> MAPTPKYTFTERAAAGNLSDAEILNSNN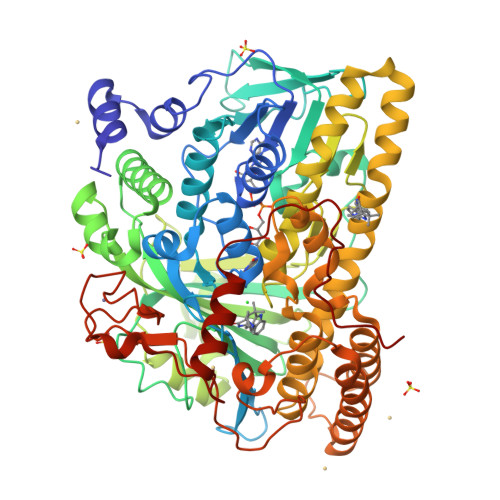PTGSELPDESDVVVGGAGIHGLIYALHASKYKPNNLKISVIEKNTRPGYKIGESTLPIFYTWCKLHGISAAYLLRLFGLKDGLCFYFLDRENQGQYTDFCSVGAPGLVLASLQIERPMSELLFTILAQRNGVNVYHGREVDFKSTVVQGGGQGNKIAVSRGKYDSTPKTIDSALFVDATGRFRQFCSKKAPRHRFDGWNCNAFWGYFTAPKDESKIPFDLYEGDATNHLCFPEGWVWVIRLPSWEGSPIANLMDMVTYILECADAGVPGDELPSSEELARMFGLKFQWVTSIGFAVRNDVKYPEDLSAYGTREAEQKFNYFVQKYELLQQFMSNFELIENLYGPGTTWFIRKTLAYQSPVVSGPGWLAIGDACGFTNPLYSPGINVGMSTSTWAAQLSHPIVEIGKSAPADAAESSIRKLLVPYDDYCKSLVPALEQMNRFNYVCYRDTRLGPQVACLWQFFAGIERYLSDVNIETFAHYAIKWVWGAMVPEYQQVAQKCIEHIETVPLDERLPDAMVDELLAFSNRIKSAAVAADDFSLRWDAILRSFDRSLNFVEGKTSRDIYTRQCSGCGAWLQLRPDWKKCHSCGLLGTEPQTAVTFDPPLTAEEEALLYAAWNTAPKYDPSKELKLPTPTRPAA> A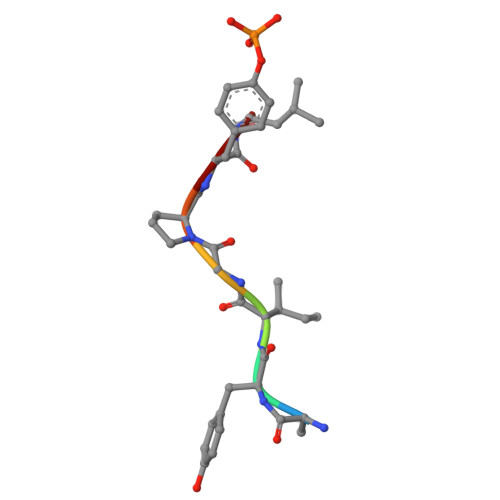YIGPYL> MRPPQFTRAQWFAIQHISLNPPRCTIAMRAINNYRWRCKNQNTFLRTTFANVVNVCGNQSIRCPHNRTLNNCHRSRFRVPLLHCDLINPGAQNISNC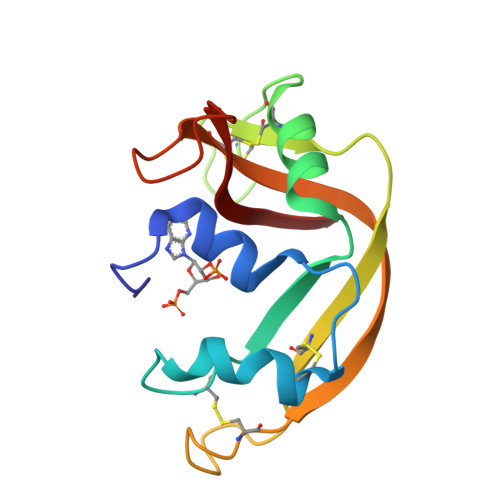RYADRPGRRFYVVACDNRDPRDSPRYPVVPVHLDTTI The final step in the pathway is catalyzed by a 2-epimerase, which utilizes UDP-2,3-diacetamido-2,3-dideoxy-d-glucuronic acid as its substrate. The focus of this investigation is on the ORF WP_011172736, which we demonstrate encodes for a 2-epimerase. We have also demonstrated that the T. thermophilus enzyme is allosterically regulated by UDP-GlcNAc. Whereas the sugar 2-epimerases that function on UDP-GlcNAc have been the focus of past biochemical and structural analyses, this is the first detailed investigation of a 2-epimerase that specifically utilizes UDP-2,3-diacetamido-2,3-dideoxy-d-glucuronic acid as its substrate.

Although UDP-GlcNAc was observed binding in structure 4, it was never included in the crystallization trials (structure 10). We reasoned that the D98N variant, for whatever reason, bound the ligand during its overexpression and purification from Escherichia coli. As a consequence, we crystallized the apoform of the D98N variant with the assumption that UDP-GlcNAc would be found in the allosteric pocket. The crystals were obtained at pH 6.0, and the model was refined to 1.8 Å resolution (overall R-factor of 18.1%). Note that the α-carbons for the apoform of the WT enzyme and the D98N variant correspond with an RMSD of 0.9 Å.

>[4x]GHMWVKILSVVGARPQFIKAAAVSRVLRASPGVREVLVHTGQHYDDNMSQVFFEELEIPDPDYHLGIGGGTHGQNTGRMLEAIEGVLLKEKPDWVLVYGNTDSTLAGALAAVKLHIPVAHVEAGLRSFNRRMPEEINRILTDHASDLLFAPTETAVQNLLREGIPENRIHLVGDVMYDAALHYGAKAERKSRILERLGLQAKGYVLATIHRAENTDDQERLRVILEALAEVHQEVPVVFPVHPRTRKRAEAFGLGSYLEKVVALEPVGYLDMVMLEKNARLIVTDSGGVQKEAYFYRVPCVTVREETEWVELLKAEWNYLAAPQNAKDLALTILHRMRTKGVEIDLYGDGRASQKISDFLRKVGIRT> MADELSTMSEPTITNHAQQQAQHLTNTELSSAESKSQDTSQITLKTNREKEQSQDLVSEPTTTELADTDAASMANTGSDATQKSASLPPVNTDVHDWVKTKGAWDKGYKGQGKVVAVIATGIDPAHQSMRISDVSTAKVKSKEDMLARQKAAGINYGSWINDKVVFAHNYVENSDNIKENQFEDFDEDWENFEFDAEAEPKAIKKHKIYRPQSTQAPKETVIKTEETDGSHDIDWTQTDDDTKYESHGMHVTGIVAGNSKEAAATGERFLGIAPEAQVMFMRVFANDIMGSAESLFIKAIEDAVALGADVINLSLGTANGAQLSGSKPLMEAIEKAKKAGVSVVVAAGNERVYGSDHDDPLATNPDYGLVGSPSTGRTPTSVAAINSKWVIQRLMTVKELENRADLNHGKAIYSESVDFKDIKDSLGYDKSHQFAYVKESTDAGYNAQDVKGKIALIERDPNKTYDEMIALAKKHGALGVLIFNNKPGQSNRSMRLTANGMGIPSAFISHEFGKAMSQLNGNGTGSLEFDSVVSKAPSQKGNEMNHFSNWGLTSDGYLKPDITAPGGDIYSTYNDNHYGSQTGTAMASPQIAGASLLVKQYLEKTQPNLPKEKIADIVKNLLMSNAQIHVNPETKTTTSPRQQGAGLLNIDGAVTSGLYVTGKDNYGSISLGNITDTMTFDVTVHNLSNKDKTLRYDTELLTDHVDPQKGRFTLTSHSLKTYQGGEVTVPANGKVTVRVTMDVSQFTKELTKQMPNGYYLEGFVRFRDSQDDQLNRVNIPFVGFKGQFENLAVAEESIYRLKSQGKTGFYFDESGPKDDIYVGKHFTGLVTLGSETNVSTKTISDNGLHTLGTFKNADGKFILEKNAQGNPVLAISPNGDNNQDFAAFKGVFLRKYQGLKASVYHASDKEHKNPLWVSPESFKGDKNFNSDI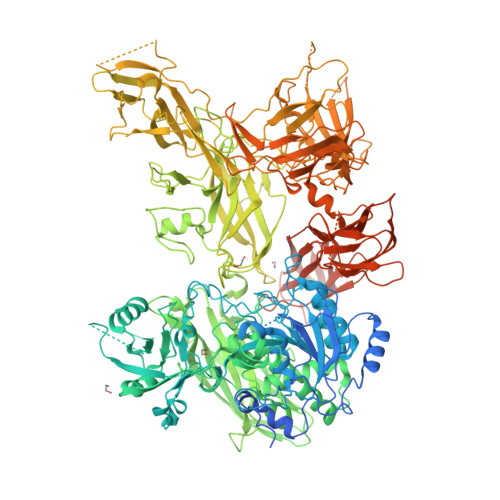RFAKSTTLLGTAFSGKSLTGAELPDGHYHYVVSYYPDVVGAKRQEMTFDMILDRQKPVLSQATFDPETNRFKPEPLKDRGLAGVRKDSVFYLERKDNKPYTVTINDSYKYVSVEDNKTFVERQADGSFILPLDKAKLGDFYYMVEDFAGNVAIAKLGDHLPQTLGKTPIKLKLTDGNYQTKETLKDNLEMTQSDTGLVTNQAQLAVVHRNQPQSQLTKMNQDFFISPNEDGNKDFVAFKGLKNNVYNDLTVNVYAKDDHQKQTPIWSSQAGASVSAIESTAWYGITARGSKVMPGDYQYVVTYRDEHGKEHQKQYTISVNDKKPMITQGRFDTINGVDHFTPDKTKALDSSGIVREEVFYLAKKNGRKFDVTEGKDGITVSDNKVYIPKNPDGSYTISKRDGVTLSDYYYLVEDRAGNVSFATLRDLKAVGKDKAVVNFGLDLPVPEDKQIVNFTYLVRDADGKPIENLEYYNNSGNSLILPYGKYTVELLTYDTNAAKLESDKIVSFTLSADNNFQQVTFKITMLATSQITAHFDHLLPEGSRVSLKTAQDQLIPLEQSLYVPKAYGKTVQEGTYEVVVSLPKGYRIEGNTKVNTLPNEVHELSLRLVKVGDASDSTGDHKVMSKNNSQALTASATPTKSTTSATAKALEHHHHHH N-(5-(6-(2-((2S,6R)-2,6-dimethylmorpholino)pyridin-4-yl)-1-oxoisoindolin-4-yl)-2-methoxypyridin-3-yl)methanesulfonamide 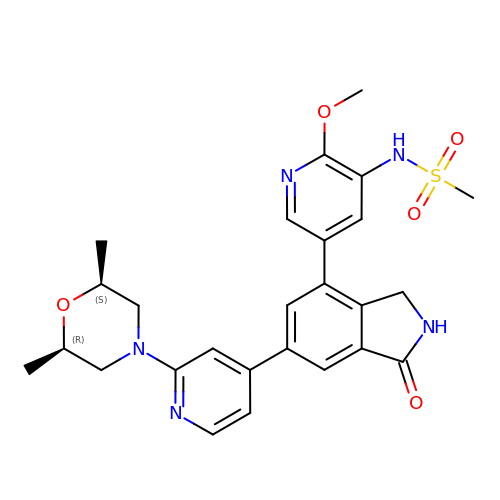| C26 H29 N5 O5 S | BTLBFTXHIOZUGF-IYBDPMFKSA-N>[2x]CPRFLKVKNWETDVVLTDTLHLKSTLETGCTEHICMGSIVLPSQHTRKPEDVRTKDQLFPLAKEFLDQYYSSIKRFGSKAHMDRLEEVNKEIESTSTYQLKDTELIYGAKHAWRNASRCVGRIQWSKLQVFDARDCTTAHGMFNYICNHVKYATNKGNLRSAITIFPQRTDGKHDFRVWNSQLIRYAGYKQPDGSTLGDPANVQF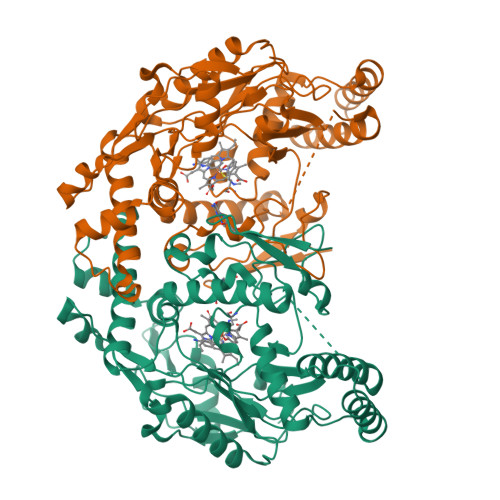TEICIQQGWKAPRGRFDVLPLLLQANGNDPELFQIPPELVLEVPIRHPKFDWFKDLGLKWYGLPAVSNMLLEIGGLEFSACPFSGWYMGTEIGVRNYCDNSRYNILEEVAKKMDLDMRKTSSLWKDQALVEINIAVLYSFQSDKVTIVDHHSATESFIKHMENEYRCRGGCPADWVWIVPPMSGSITPVFHQEMLNYRLTPSFEYQPDPWNTHVWKG>MAGKSPEEEHPVKAYGWAVKDRTTGILSPFKFSRRATGDNDIRIKILYCGICHTDLTSVKNEYEFLSYPLVPGMEIVGIATEVGSKVTKIKVGEKVAVAAYLGTCGKCYNCVNDLENYCPEVIIGYGTPYHDGTINYGGLSNETVVNERFVLRFPEKLSPAGGAPLLSAGITAYSAMRNHGLDKPGIHLGVVGLGGLGHLAVKFAKAFGVRVTVISTTPSKKDEAINNLGADAFLFSRDDKQMRAAIGTFDAIIDTLAVVHPIAPLLDLLRSHGKLVLVGAPSKPLELPT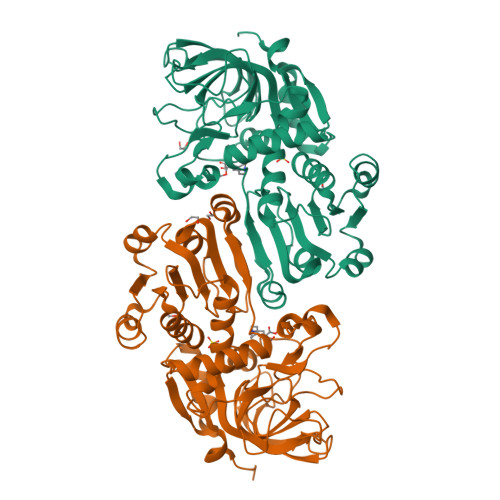IPLLSGGKSLIGSAAGNVKQTQEMLDFAAEHDITANIEVIPIDYINTAMERLDKGDIRFRFVVDIENTLTPPPEP[2x]> EAVTDHPDRLWAWEKFVYLDEKQHAWLPLTIEIKDRLQLRVLLRREDVVLGRPMTPTQIGPSLLPIMWQLYPDGRYRSSDSSFWRLVY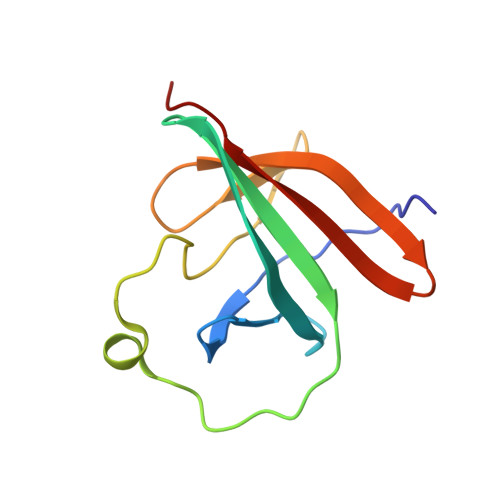HIKIDGVEDMLLELLPDD> MADPSSSTSAMPLDEIQWHTNPAVVGGSIHDNSVLFYFRESPFYDKTSNNEVLYQQGLHNQTMMQFLETRERFERRLREMSGLE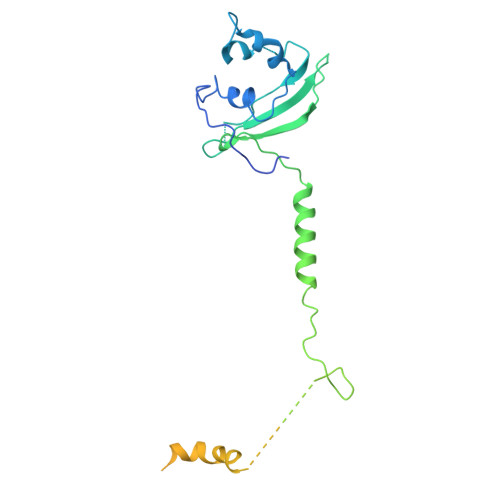FVVAQEPAETAPGTGTGVWVINKQTRRKRQGEEDEISVHGTYFLVGENVYMAAPTLADIISMRLASASSSISRLLPIAASVQSWSPGTGRVYKTPSMTSQTNQANQPSSQTQSQPTSQPATTTTTTALPPPDPRWLEETLMIHEFFGDHHLDKNPITGKPGDFHLSSTGRKIQTLPTAAAGNKKPGSGLPPLPAINTKVQQNPMGSGKQVTGKETKSPKTPSSSTGPGTGGMSTGMGKPKKRKSSKAAVTPTS> MNARSTGQHPARYPGAAAGEPTLDSWQEPPHNRWAFAHLGEMVPSAAVSRRPVNAPGHALARLGAIAAQLPDLEQRLEQTYTDAFLVLRGTEVVAEYYRAGFAPDDRHLLMSVSKSLCGTVVGALVDEGRIDPAQPVTEYVPELAGSVYDGPSVLQVLDMQISIDYNEDYVDPASEVQTHDRSAGWGTRRHGDPADTYEFLTTLRGDGSTGEFQYCSANTDVLAWIVERVTGLRYVEALSTYLWAKLDADRDATITVDTTGFGFANGGVSCTARDLARVGRMMLDGGVAPGGRVVSEDWVRRVLAGGSHEAMTDKGFTNTFPDGSYTRQWWCTGNERGNVSGIGIHGQNLWL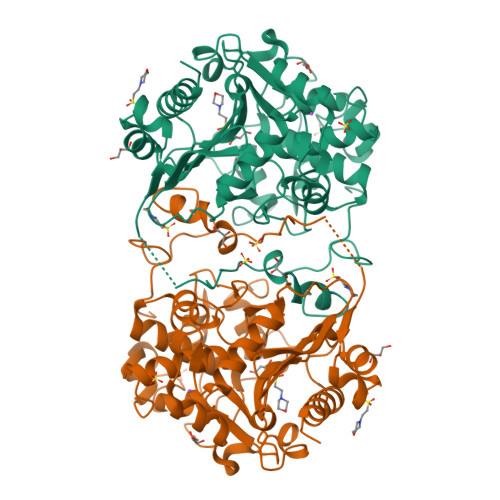DPLTDSVIVKLSSWPDPYTEHWHRLQNGILLDVSRALDAV> MGHHHHHHHHHHSSGHIDDDDKHMPAHASPFNAPSSASRAGAARLGTSRRFAPFVLAALAILMGAMSVVALCVGAYRIPLAEAWAALSGDPAAQQARAVLLDIRAPRV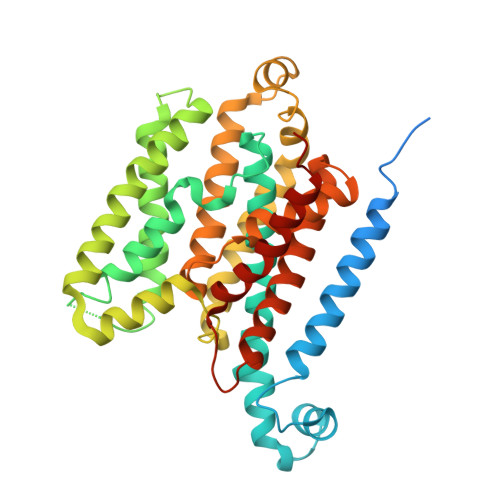VLALLVGGGFGATGAAMQALFRNPLADPGLVGVSSGAALGATTLIVLGPALFAAHASAAALPVAAFAGGLAVAALVYRLAASRGRLALPLLLLAGIAINALVGAAIGLLTFVADDAQLRSLTFWSLGSLGGAQWPTLAAVAPCVALGGVLLVRERDALNALQLGETEALHLGVPVQRLKRRVLVAVALAVGALVSCAGIIGFIGLVAPHCVRLACGPDQRIVLPGAALLGALLTLAADLAARTVAAPADIPLGVLTALLGAPFFLALLWKNRGALGG> MQIYHTDVLCIGGALAGERVAVEASMAGLKTIMLSLVPPRRSHSSAAQGGMQAAL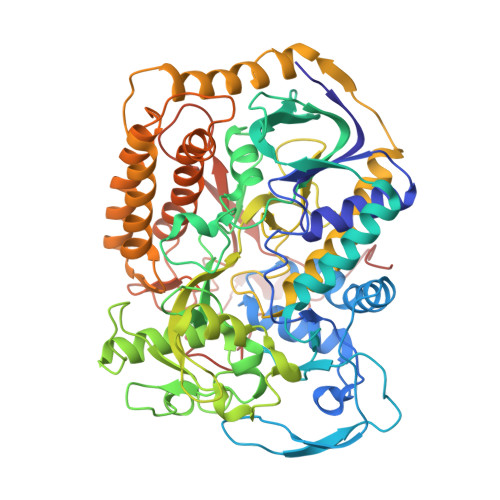GNAIMGDGDSPDVHFADTVKGSDWGCDQEVARIFADTAPIVMREVAHWGVPWNRVVPGKHTYYKGGKPFEAEEKAEKAGLIHARAFGGTAAWRTCYTADGTGRSVLNTLDTKCLQYGVTVHDRMQAEALIHDGGNCLGCIARCLRTGELVAYLATSTLIATGGYGRIYKATTNAVICDGGGQIIALDTGLVPMGNMEAVQFHPTGTVPTDILVTEGCRGDGGTLLDVNQYRFMPDYEPDKAQLASRDVVSRRMTEHMRKGLGVKSPYGDHLWLDIRHLGEKHITTKLREVYDICTNFLGVNPIHQLIPVRPTHHYSMGGVRTNRDGAAYGLKGLFSAGESACWDMHGFNRLGGNSLAETVVAGRYIGERMVEFTKGATPSFGMQYVEDAHKKVQERITDIVTGRKGKENTFKIRDEMHDIMMEGVGIFRNGTDLQKAVNKLEELYDRSQKISLSSACKGMNPELSTALRIRGMLKLAQCTAYGALDRTESRGAHTREDFPERNDKEWLNRTLSYWKEGASMPTLEYEEASPYYEMPPGDRGYGGGVTIANELPPEKFVIPEAAKENLKKAKL>[2x]GSHMMERAESSSTEPAKAIKPIDRKSVHQICSGQVVLSLSTAVKELVENSLDAGATNIDLKLKDYGVDLIEVSDNGCGVEEENFEGLTLKHHTSKIQEFADLTQVETFGFRGEALSSLCALSDVTISTCHASAKVGTRLMFDHNGKIIQKTPYPRPRGTTVSVQ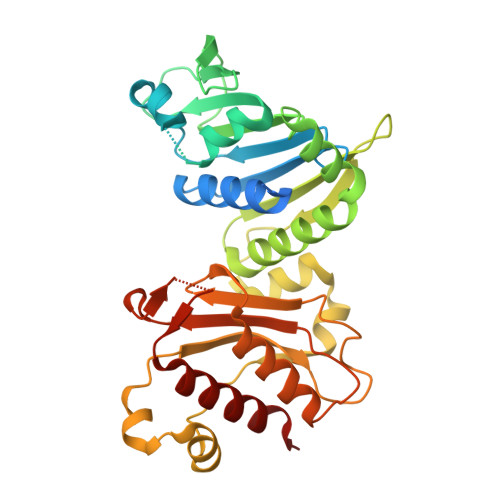QLFSTLPVRHKEFQRNIKKEYAKMVQVLHAYCIISAGIRVSCTNQLEQGKRQPVVCTGGSPSIKENIGSVFGQKQLQSLIPFVQLPPSDSVCEEYGLSCSDALHNLFYISGFISQCTHGVGRSSTDRQFFFINRRPCDPAKVCRLVNEVYHMYNRHQYPFVVLNISVDSECVDINVTPDKRQILLQEEKLLLAVLKTSLIGMFDS> MNFSSSARWLAVRQSQTLGHTTRATVAAGRRVLAHSPAATEFTSFQSLHIGGDVCKLPLAVALGAAPSALGYGSAKHNQQRQYATLGSGWSFSKVQYTKYRITKPWTTDTTFDDIILSQPSKEDFAKFTKEAPLFLRFLKLVTDVEGRQEAFIQFAKRCENGLT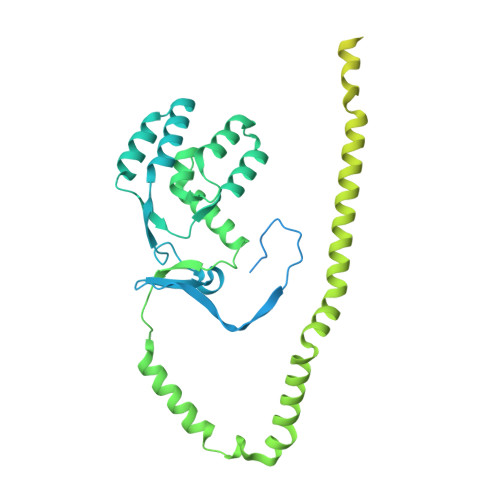VEKDVYVTKKELVDCLWKNGYTDTEINAFEIAFPADYKFHYPELAVLFDLTEEDCYKYCIRQRAATPEELVELKYTKPKNLVSSYGLCFLGVWFGLSNTVLSNAWFYSKTFPFGAVFYMLGSYFYRDIREKLWKEEKSLIHTAQENKNMGEESVYKQMKKYATDTKCLDYLSTFRTEVEDQIANYKVALVSQMRRQLTERLVEKLNGIQQAEKLIQGSLQDVMIREIVSSFKDLYKSRPELHDAAMQSAIQGLSGSDGAMDPVGAHFKASLQELAKVNLSTATADPMGTVVQRVAAVFQKREKEFLDTFTVKATEAQEIKTIVDKCHKGNTFDFHALSDEELRRLEQLYSTVNNRVGFETIHENSIKPVAPLSENSKGFVEFVNTQLEITKAKLRNARLTAFAHAFV> GPMPSPLLSTHNVTVLGNRSDPVVVLGHGLGTDQSVWKYTVPSLVNQNFQVVLYDTMGAGSTETSDFNFKRYSSLQGHVDDLLAILDELEIENCVYVGHSMSGMIGVLASLERPDLFRKLILLSASPRYLNDSSYYGGFEQEDLDQLFSSMRSNFSAWVSGFATAAVGTDIHDEAVQEFSSTFISMRPD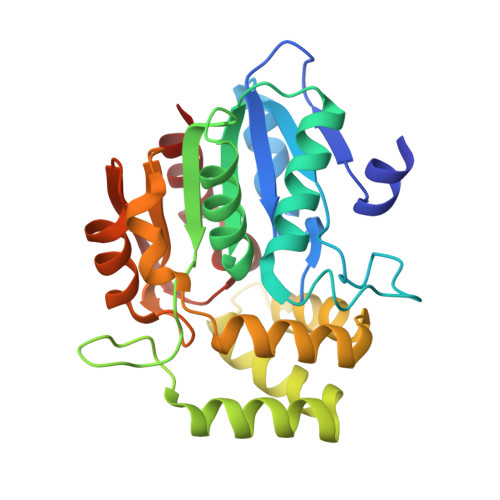VALRTSQFVFQSDFRSILSEVTVPCHIVQSRKDIAVPIEVAEYLRCNLGGWTSVDILQTDGHLPQLSCPELVVPVLLHCIDS>MVSKGEELIKEEMPMKVVLEGTVNGHQFKCTGEGEGRPYEGVQTMRIKVIEGGPLPFAFDILATSFMYGSRTFVKHPKGIPDYFKQSFPEGFTWERVMRFEDGGVVTVTQDTSLQDGVLIYNAKVRGVNFPSNGPVMQKKTKGW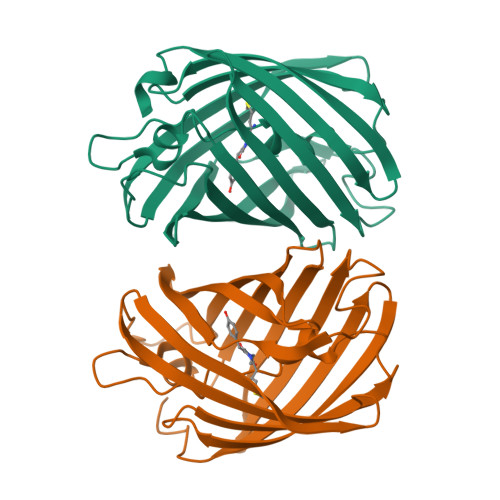EPNTEMIYPADGGLRGYTDMALKVDGGGHLHCSFVTEYRSKKTVGNIKMPGVYAIDHRLERIEESDNETYVVQREVAVAKYSNLGGGMDELYK[2x]>[2x]ELIRVAILWHEMWHEGLEEASRLYFGER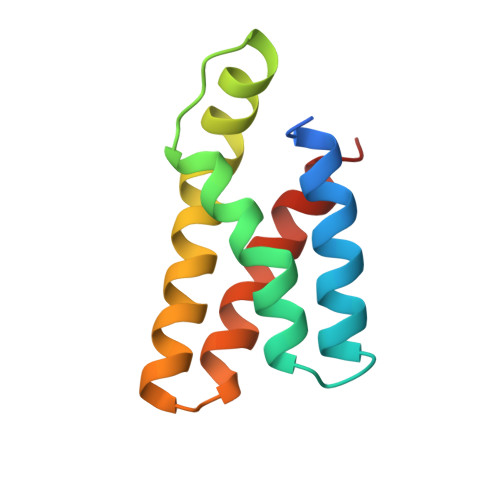NVKGMFEVLEPLHAMMERGPQTLKETSFNQAYGRDLMEAQEWCRKYMKSGNVKDLTQAWDLYYHVFRRISKQ> MKLTRRAFLQVAGATGATLTLAKNAMAFRLLKPAVVVDNPLDTYPDRRWESVYRDQYQYDRTFTYCCSPNDTHACRIRAFVRNNVMMRVEQNYDHQNYSDLYGNKATRNWNPRMCLKGYTFHRRVYGPYRLRYPLIRKGWKRWADDGFPELTPENKTKYMFDNRGNDELLRASWD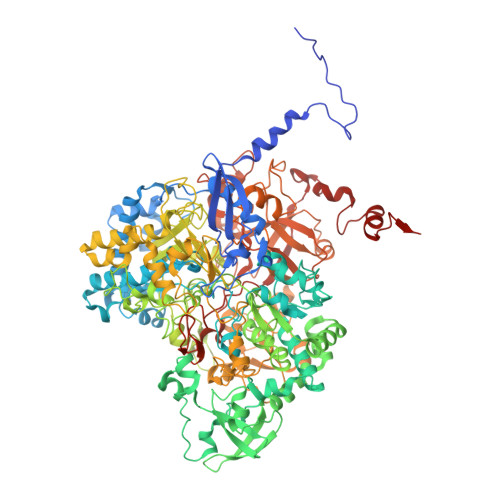EAFTYASKGIIHITKKYSGPEGAQKLIDQGYPKEMVDRMQGAGTRTFKGRGGMGLLGVIGKYGMYRFNNCLAIVDAHNRGVGPDQALGGRNWSNYTWHGDQAPGHPFSHGLQTSDVDMNDVRFSKLLIQTGKNLIENKMPEAHWVTEVMERGGKIVVITPEYSPSAQKADYWIPIRNNTDTALFLGITKILIDNKWYDADYVKKFTDFPLLIRTDTLKRVSPKDIIPNYKLQDISDGPSYHIQGLKDEQREIIGDFVVWDAKSKGPKAITRDDVGETLVKKGIDPVLEGSFKLKTIDGKEIEVMTLLEMYKIHLRDYDIDSVVSMTNSPKDLIERLAKDIATIKPVAIHYGEGVNHYFHATLMNRSYYLPVMLTGNVGYFGSGSHTWAGNYKAGNFQASKWSGPGFYGWVAEDVFKPNLDPYASAKDLNIKGRALDEEVAYWNHSERPLIVNTPKYGRKVFTGKTHMPSPTKVLWFTNVNLINNAKHVYQMLKNVNPNIEQIMSTDIEITGSIEYADFAFPANSWVEFQEFEITNSCSNPFIQIWGKTGITPVYESKDDVKILAGMASKLGELLRDKRFEDNWKFAIEGRASVYINRLLDGSTTMKGYTCEDILNGKYGEPGVAMLLFRTYPRHPFWEQVHESLPFYTPTGRLQAYNDEPEIIEYGENFIVHREGPEATPYLPNAIVSTNPYIRPDDYGIPENAEYWEDRTVRNIKKSWEETKKTKNFLWEKGYHFYCVTPKSRHTVHSQWAVTDWNFIWNNNFGDPYRMDKRMPGVGEHQIHIHPQAARDLGIEDGDYVYVDANPADRPYEGWKPNDSFYKVSRLMLRAKYNPAYPYNCTMMKHSAWISSDKTVQAHETRPDGRALSPSGYQSSFRYGSQQSITRDWSMPMHQLDSLFHKAKIGMKFIFGFEADNHCINTVPKETLVKITKAENGGMGGKGVWDPVKTGYTAGNENDFMKKFLNGELIKVDA(4-hydroxyphenyl)-[2,3,4-tris(oxidanyl)phenyl]methanone | C13 H10 O5 | 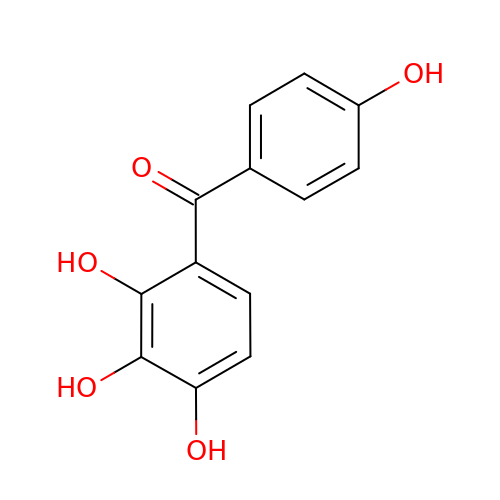ZRDYULMDEGRWRC-UHFFFAOYSA-N>ETGDEDLP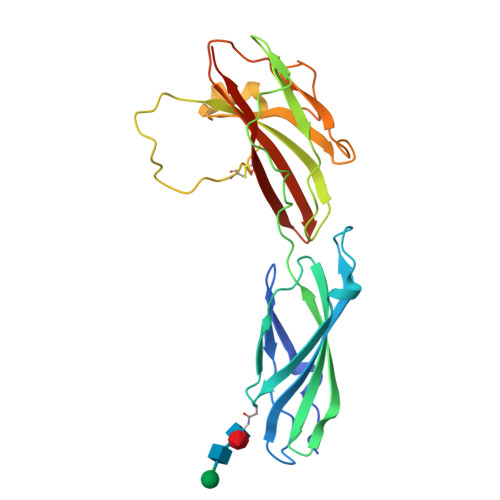GAVPTESIQGSTFEEKIFLQWREPTQTYGVITLYEITYKAVSSFDPEIDLSNQSGRVSKLGNETHFLFFGLYPGTTYSFTIRASTAKGFGPPATNQFTTKISAPSMPAYELETPLNQTDNTVTVMLKPAHSRGAPVSVYQIVVEEERPRRTKKTTEILKCYPVPIHFQNASLLNSQYYFAAEFPADSLQAAQPFTIGDNKTYNGYWNTPLLPYKSYRIYFQAASRANGETKIDCVQVATKGGTKHHHHHH[4x]> MDLNSKKYQMLKELYVSFAENEVKPLATELDEEERFPYETVEKMAKAGMMGIPYPKEYGGEGGDTVGYIMAVEELSRVCGTTGVILSAHTSLGSWPIYQYGNEEQKQKFLRPLASGEKLGAFGLTEPNAGTDASGQQTTAVLDGDEYILNGSKIFITNAIAGDIYVVMAM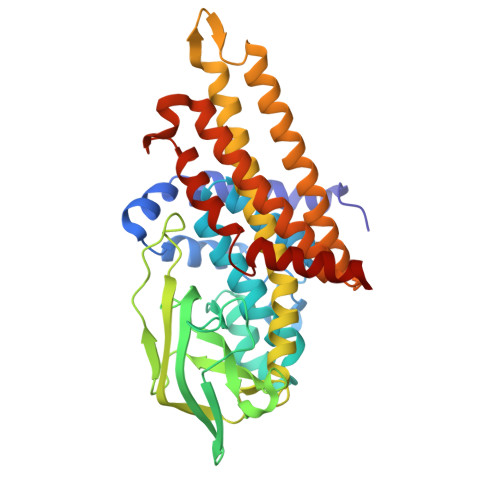TDKSKGNKGISAFIVEKGTPGFSFGVKEKKMGIRGSATSELIFEDCRIPKENLLGKEGQGFKIAMSTLDGGRIGIAAQALGLAQGALDETVKYVKERVQFGRPLSKFQNTQFQLADMEVKVQAARHLVYQAAINKDLGKPYGVEAAMAKLFAAETAMEVTTKAVQLHGGYGYTRDYPVERMMRDAKITEIYEGTSEVQRMVISGKLLK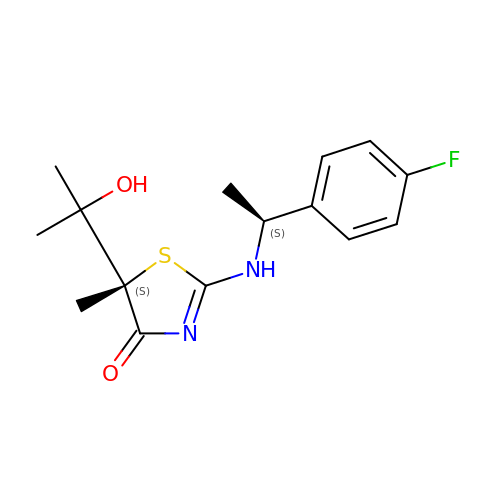(5S)-2-{[(1S)-1-(4-fluorophenyl)ethyl]amino}-5-(1-hydroxy-1-methylethyl)-5-methyl-1,3-thiazol-4(5H)-one | C15 H19 F N2 O2 S | HYVZYASDRIAOPU-BJOHPYRUSA-N> MKTNLKNNIMKGMAVMPFLSVCVGVAAQQKQMNVIYIMSDDHTSQAIGAYGSRLAVLNPTPTIDELA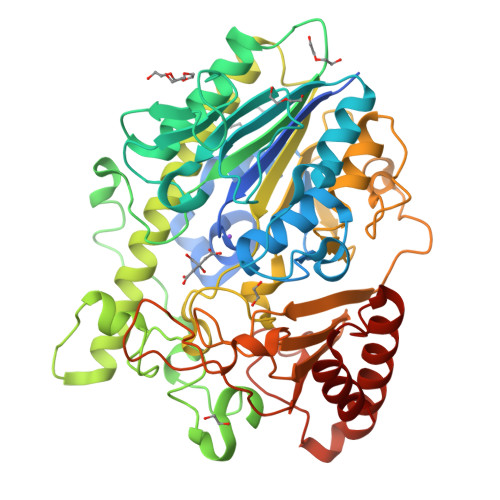RDGMLFENCFCTNSISTPSRACIMTGQYSHRNKVLTLDEVLQPDQEYLVDEFHNMGYQTAMIGKWHLGCEPSHFDYYSVFNGHGGQGEYFDPTFLTSDVTDKKWPNNQIKKMGYSSDIVTNLAIDWLKNRRDKSKPFFMMHHYKAPHDMFEYAPRYEYYLDDVEVPVPLSLFDTDKWGSEGTRGKNDSLRHFIGTSVSSRHEIRNYVMEYKCNTGDEMENTYLAYQHYLKSYLRCVKGVDDNLKRLFDYLKKEGLWENTIIVYTGDQGMMLGEHDLQDKRWMYEESQRMPFIVRDPRCPYKGAKSDLMINNIDFAPTLIEMVGGKEPSYMDGKSFASVFEGKKPENWKDAVYYRYWMHMIHHDVPAHIGIRTENYKLILFYGRHYDDKRYGQKSMSWLKNSHKIVPTLVSFELYDVKNDPYEMVNLADNPKYAKVLKDMKKKLRELRKQVGDTDEAYPELKKVIDKALR>SDKKSLMPLVGIPGEIKNRLNILDFVKNDKFFTLYVRALQVLQARDQSDYSSFFQLGGIHGLPYTEWAKAQPQLHLYKANYCTHGTVLFPTWHRAYESTWEQTLWEAAGTVAQRFTTSDQAEWIQAAKDLRQPFWDWGYWPNDPDFIGLP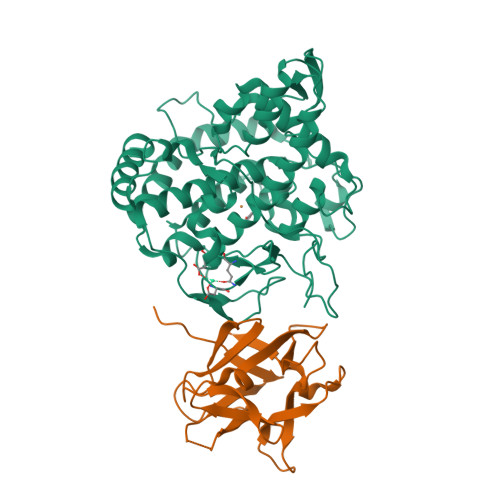DQVIRDKQVEITDYNGTKIEVENPILHYKFHPIEPTFEGDFAQWQTTMRYPDVQKQENIEGMIAGIKAAAPGFREWTFNMLTKNYTWELFSNHGAVVGAHANSLEMVHNTVHFLIGRDPTLDPLVPGHMGSVPHAAFDPIFWMHHCNVDRLLALWQTMNYDVYVSEGMNREATMGLIPGQVLTEDSPLEPFYTKNQDPWQSDDLEDWETLGFSYPDFDPVKGKSKEEKSVYINDWVHKHYG[4x];>[4x]MAQARKIPLDLPGTRILNGANWANNSATENLATNSGTLIIFDQSTPGQDADRWLIHNYLDGYKIFNMGSNNWASVSRGNTVLGVSEFDGQTCKWSIEYSGNGEEFWIRVPREGGGGAVWTIKPASSQGPTTVFLDLLKETDPNQRIKFAV> GMDVNVRGPDGFTPLMIASCSGGGLETGNSEEEEDAPAVISDFIYQGASLHNQTDRTGETALHLAARYSRSDAAKRLLEASADANIQDNMGRTPLHAAVSADAQGVFQILIRNRATDLDARMHDGTTPLILAARLAVEGMLEDLINSHADVNAVDDLGKSALHWAAAVNNVDAAVVLLKNGA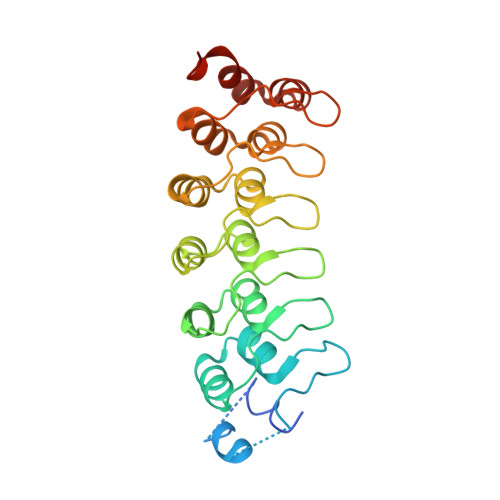NKDMQNNREETPLFLAAREGSYETAKVLLDHFANRDITDHMDRLPRDIAQERMHHDIVRLLDEYNLVRSPQLHG> MKKVMLATALFLGLTPAGANAADLGHQTLGSNDGWGAYSTGTTGGSKASSSNVYTVSNRNQLVSALGKETNTTPKIIYIKGTIDMNVDDNLKPLGLNDYKDPEYDLDKYLKAYDPSTWGKKEPSGTQEEARARSQKNQKARVMVDIPANTTIVGSGTNAKVVGGNFQIKSDNVIIRNIEFQDAYDYFPQWDPTDGSSGNWNSQYDNITINGGTHIWIDHCTFNDGSRPDSTSPKYYGRKYQHHDGQTDASNGANYITMSYNYYH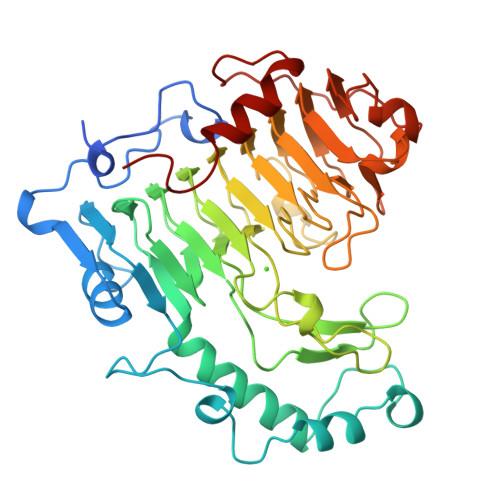DHDKSSIFGSSDSKTSDDGKLKITLHHNRYKNIVQRAPRVRFGQVHVYNNYYEGSTSSSSYPFSYAWGIGKSSKIYAQNNVIDVPGLSAAKTISVFSGGTALYDSGTLLNGTQINASAANGLSSSVGWTPSLHGSIDASANVKSNVINQAGAGKLN> MMRRVASTGSNGGHCYVGSSLWADSVYMEVSSITLQKRFSFKYATKLQHDEMRQPYYIHEKRYGIFSNERNIAKARRGLPFITPLYTKHMNLWDTDTDASNNRFFRGYYYGQRELHQLLGRPHSLEATNADGSNDLSTYEANTSQLYKGIPRPAITNLHYEPAWRYTLYQAGAHGAQLSNPRSPFTAKVLGDELMQVRDIKSVEHCKAWFDRLQYLINLHYEAVGDIGEFKSRHTRHVHEFFVAFHDALSSLDFRDTYLFDQFKAVRPPELSDLFGIFLEMEANYVHEDYCPRCSLPYSTTRYCGEGDVDTPFRKHRGRWAPHQKWGREWYDVVARRAEALWYRATEDPYFGTPQHTQRQAEALLKVYVQAKQRGKAIDFMNKLRGSVEYLTGDITITTVMQESYDALLDTTPHPHLLTNGFTLESDAAKYTGEVNKAPLSPLQFRIDMEMNKYRRQQKEEGVVRVPPALWRLDTSAIVPYKVDSKTRRIVNWREVKEGIEKSFLSVGLPKEAYTGNEWREMLYLHDVIANREAKAAVLEQQQKLDREKLKARERASLKGEKSSNSASNGIGIIFPDKDGYQVFFVDEASLRPFGIGASGTLFKAVARVYPSPAAVP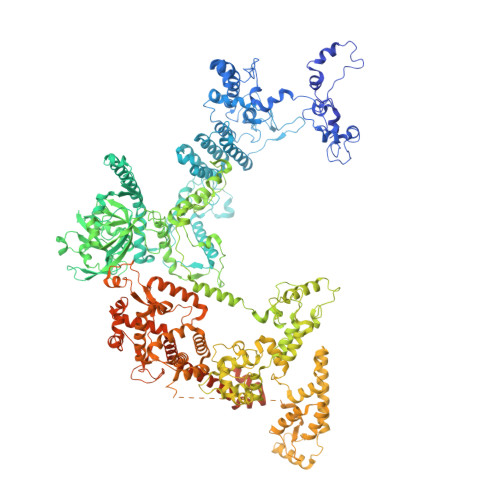YDDPVHGKQFLIDTTDETCHLFGGFEHGDRLLLRAKSSGGDVDGGNNSNCRNTGSFTDEEEEVIVMGVSTEGSDAERMLCAMHVDTGKQRERGIVFLGTDCIDIRERWESVRYAASAYVKGRVTLLESQRTAREEFMGQVVGIRDGVLFVQWRLLKGGGSVLDRSVAVPIGDSTQVRELFVETKVLGVEPLQSPPSWRTPFRNDFAEERLKELQRAPFKREKYVSLIQGKYTPKVKKFGYTQHTTVDDFETKEYKDRLLSKQFFQNPQAFEVVPDRNERSVQFGGKWEYQRTHGLPTVDRNELENGWSEVEPISDGEMKVIEQALRDISGPRPGNFVKPPSKTKSLQLSESWWEPLGYGWEQHNEEQKALCDVTEQRLIDGSNLPFGGKLPPFGTSYGMGERMRAIIEDYSKGFGLGPHGHSPTHDTIHYNTLNAEGERVRDLGYTDALGRLFSEKLGDRDVHQWAVESCADGEADVRQLLLSLHEWRERGRPPSLLLANVLSKYLEEEIAAFNKGIPENAPKLQLETSDGTLAHSGSGGSRSGTMWADVDPTTFALHQASQSTRSTRCDEPFILHLVKRAKLGECVTNFTDTAYIAHLESSVINEFHLALTKLVGKGISPTLLAQKTGQLHRGSVRVGGNVVPFVKSRELSRLLERMGLTSESIAVITRGLANCPEQESVGDDFAVPVSLILSWDGPGSSGGSGSGDRRLNTTAARNEQQRKGSAALSSAIRQLSQHQKQRGSASGRGWQNEDKMVVHVLEELSLRNDGLVMDIQYAIRENKKNRRLRWEFVTTLLPVFGGNEAKVEQLYSDYCDGKYVPNITVAVEAFIAFLHNATQHPETYSASDYFDIDDGKSSTASGTGDQPSAGQYTTLKLLDPLEGPFVFDNVKVEYIQTVERFRRHGIRAGPVMAPATGFIAANCKSLNYFTRRQEEVVYVTNDSDQGLRRSLENSAYHKTIAANPALQYLLKARRGAALVETFNRFFYRTMPMLNFYQNVLKHYSETIQPLRQAAKSSTRGLARALESERSAAMEEFRRNSERYWRNIIEGRSVEQVVLANGESNRRTVGGGAGEQLQKPQGNRDAVRTNFTGEATDGSRKGQRQHQQPPLSQQQQHSRGEGERSAVHTSPRQGGSRGMADLLSKLNTPKTGSGVKGSTAKNTGNNRRGPKS> MVTFHTNHGDIVIKTFDDKAPETVKNFLDYCREGFYNNTIFHRVINGFM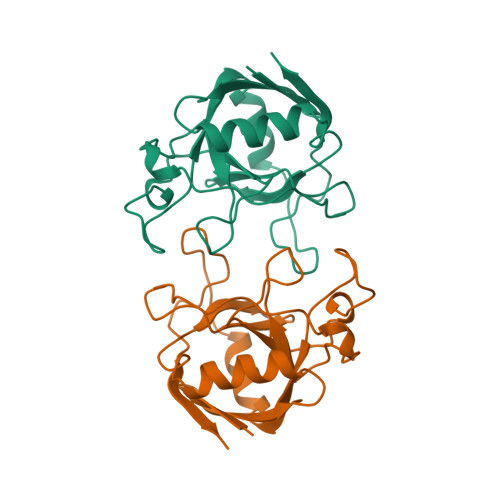IQGGGFEPGMKQKATKEPIKNEANNGLKNTRGTLAMARTQAPHSATAQFFINVVDNDFLNFSGESLQGWGYCVFAEVVDGMDVVDKIKGVATGRSGMHQDVPKEDVIIESVTVSE> MTLEKFVDALPIPDTLKPVQQSKEKTYYEVTMEECTHQLHRDLPPTRLWGYNGLFPGPTIEVKRNENVYVKWMNNLPSTHFLPIDHTIHHSDSQHEEPEVKTVVHLHGGVTPDDSDGYPEAWFSKDFEQTGPYFKREVYHYPNQQRGAILWYHDHAMALTRLNVYAGLVGAYIIHDPKEKRLKLPSDEYDVPLLITDRTINEDGSLFYPSAPENPSPSLPNPSIVPAFCGETILVNGKVWPYLEVEPRKYRFRVINASNTRTYNLSLDNGGDFIQIGSDGGLLPRSVKLNSFSLAPAERYDIIIDFTAYEGESIILANSAGC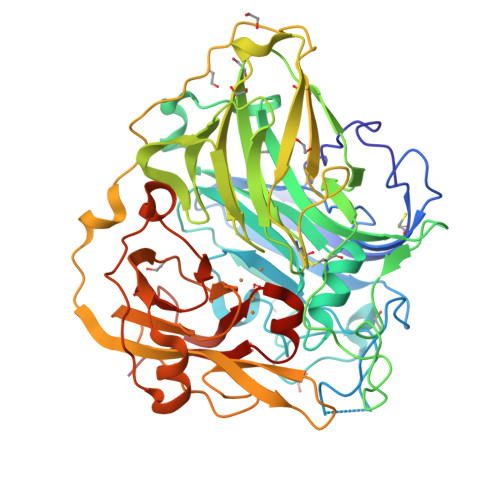GGDVNPETDANIMQFRVTKPLAQKDESRKPKYLASYPSVQHERIQNIRTLKLAGTQDEYGRPVLLLNNKRWHDPVTETPKVGTTEIWSIINPTRGTHPIHLHLVSFRVLDRRPFDIARYQESGELSYTGPAVPPPPSEKGWKDTIQAHAGEVLRIAATFGPYSGRYVWHCHALEHEDYDMMRPMDITDPHK N-(3,5-dichloro-4-{[6-(methylamino)pyrimidin-4-yl]oxy}phenyl)-N'-[3-(trifluoromethyl)phenyl]urea 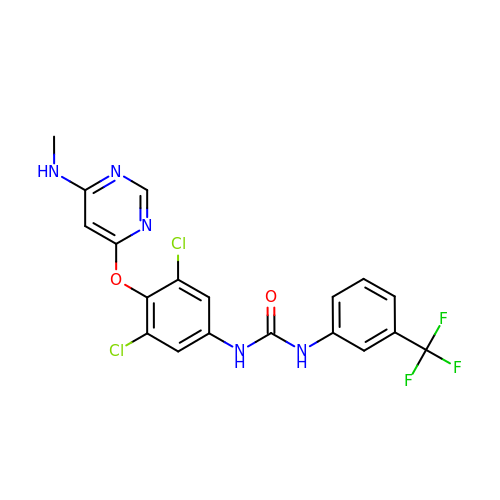| C19 H14 Cl2 F3 N5 O2 | QOQADIYOLOHRAW-UHFFFAOYSA-N> MGLIKKVTHWSYDNLIDYLSVNPTRDEVTHYKVDPENESDESIIKLHTVKDFGSITCLDYSESEIGMIGVGEKNGYLRIFNISGQNSSSPASHAPVGLNANNETSMTNASGGKAAQAENIVGSVSNLKDTQGYPVSETNYDIRVRAKKQRCINSLGINTNGLIAMGLDRNKHDSSLQIWDMNYHDDSHETINPMFSYCTNESIVSLKFLNDTSVLAASTKFLKEIDVRSPNPIYQHPTRLTYDIKLNPFNDWQFSTYGDDGTLAIWDRRKLSDQASLGDLNVASPLLTFEKLVGSGAASRKYMNSCFRWSCVRNNEFATLHRGDTIKRWRLGYYCDSNRDIAADDDNEMNIENLFVSSVHDTNTMYDRVATFDYIPRSNNGTSLICMRQSGTIYRMPISEVCSKAILNNRNSLLLSNFENTEIDEI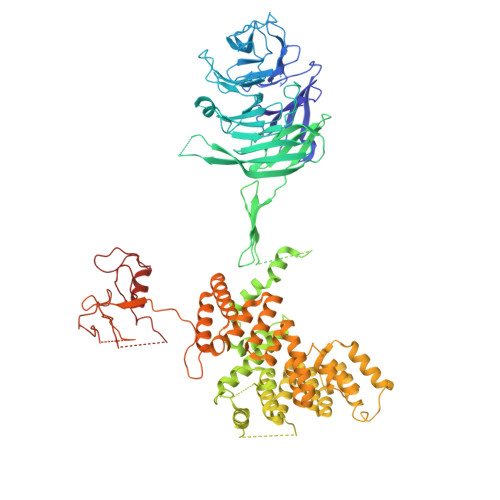RVNNEHEKSNLENVKTILKNLSFEDLDVSEDYFPSGHDEPNNEIEYSELSEEENEGSNDVLDSKRGFELFWKPEKLLEKDISVIMRTRASLGYGLDPMNTVEMIDSSKNLQNNAYIRNTWRWIAIAKASVDDGTMVSGDLDLGYEGVIGIWNGINGISNQDRYRQETILSDKQLNKEMEKIIKLRRKNRDRNSPIANAAGSPKYVQRRLCLIISGWDLSRSDYEDKYNIIMKNGHYEKAAAWAVFFGDIPKAVEILGSAKKERLRLIATAIAGYLAYKDLPGNNAWRQQCRKMSSELDDPYLRVIFAFIADNDWWDILYEPAISLRERLGVALRFLNDTDLTTFLDRTSSTVIENGELEGLILTGITPNGIDLLQSYVNKTSDVQSAALISIFGSPRYFRDQRVDEWIQTYRDMLKSWELFSMRARFDVLRSKLSRTKTGVLTADIKPRQIYIQCQNCKQNINTPRTSSPSSAVSTSAGNYKNGEAYRRNNADYKKFNTGSSEAQAADEKPRHKYCCPHCGSSFPRCAICLMPLGTSNLPFVINGTQSRDPMQTEDSQDGANRELVSRKLKLNEWFSFCLSCNHGMHAGHAEEWFDRHNVCPTPGCTCQCNK>[2x]MTKENICIVFGGKSAEHEVSILTAQNVLNAIDKDKYHVDIIYITNDGDWRKQNNITAEIKSTDELHLENGEALEISQLLKESSSGQPYDAVFPLLHGPNGEDGTIQGLFEVLDVPYVGNGVLSAASSMDKLVMKQLFEHRGLPQLPYISFLRSEYEKYEHNILKLVNDKLNYPVFVKPANLGSSVGISKCNNEAELKEGIKEAFQFDRKLVIEQGVNAREIEVAVLGNDYPEATWPGEVVKDVAFYDYKS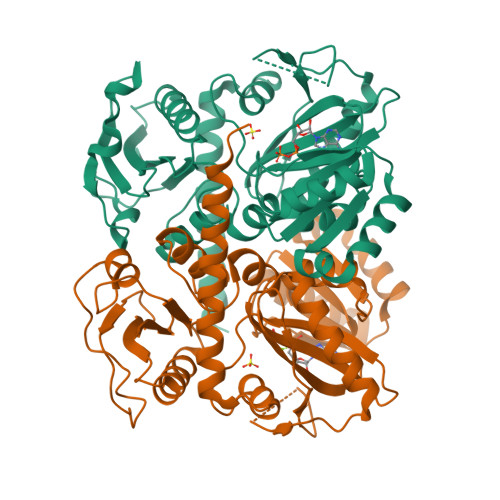KYKDGKVQLQIPADLDEDVQLTLRNMALEAFKATDCSGLVRADFFVTEDNQIYINETNAMPGFTAFSMYPKLWENMGLSYPELITKLIELAKERHQDKQKNKYKIDRSHHHHHH> DVGSVIDASLFDQLLKHRNDPACEGKGFYSYNAFVTAARSFGGFGTTGDTNTRKREVAAFLAQTSHETTGGAAGSPDGPYAWGYCFVTERDKSNKYCDPGTPCPAGKSYYGRGPIQLTHNYNYAQAGRALGVDLINNPDLVARDAVISFKTAIWFWMTPQGNKPSCHDVITNRWTPSA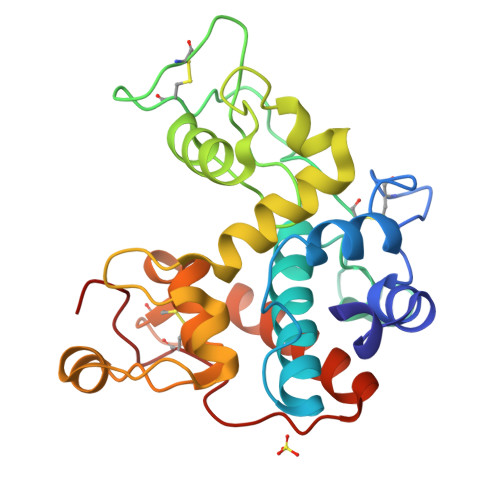ADVAANRTPGFGVITNIINGGIECGRGPSPASGDRIGFYKRYCDVLHLSYGPNLNCRDQRPFGG>[2x]GPLGSKNHTLYDGQSNGEAKVKKIEFSEFTVKIKNKNNSNNWADLGDLVVRKEEDGIETGLNVGKGDSDTFAGYTATFFSLEESEVNNFIKAMTEGGSFKTSLYYGYKDEQSNANGIQNKEIITKIEKIDDFEYITFLGDKIKDSGDKVVEYAILLEDLKKNLK

The bacterium utilizes a set of proteins, termed complement regulator-acquiring surface proteins (CRASPs), to aid evasion of the human complement system by recruiting and presenting complement regulator factor H on its surface in a manner that mimics host cells. Another member of the CRASP family, ErpC (also referred to as BbCRASP-4), is an 18 kDa protein that belongs to the OspE/F-related (Erp) paralogous family of proteins and has also been demonstrated to bind factor H. Moreover, ErpC has been implicated in the scavenging of complement factor H-related proteins CFHR-1, CFHR-2 and CFHR-5, although the functional implications of this ability to bind multiple complement proteins has yet to be fully understood. ErpC is a member of the CRASP family of proteins which aid in complement evasion by B. burgdorferi by binding and presenting complement factor H on the bacterial cell surface under distinct circumstances.

The atomic resolution structure of ErpC has been solved, showing the formation of a β-­barrel, an architecture which is completely different to the pre­dominantly α-helical CspA, which is the only other member of the CRASP family for which the structure has been elucidated. Several of the loops between β-strands could not be built in one or both copies of ErpC in the unit cell owing to a lack of electron density, suggesting that these regions are conformationally labile. However, ErpC lacks the additional structural elements that are involved in these assemblies, suggesting that it does not multimerize in a similar manner, and analysis of the interfaces between the ErpC molecules in the crystal using PISA suggested that there were no biologically relevant assemblies. The observed molecular mass of 17 000 Da correlated with the expected molecular mass of ErpC (18 316 Da), confirming that the protein is monomeric under these conditions and, in conjunction with the PISA analysis, that it is likely to be monomeric on the spirochete surface. The solvent-accessible surface of ErpC exhibits large regions of negative charge, which suggests that ErpC may be acting in a similar capacity by binding factor H via interaction interfaces reserved for host-cell localization. The binding site of complement regulators on ErpC is likely to involve residues within the loops between the β-strands in a similar manner to other bacterial factor H-binding proteins. Mapping the sequence conservation between ErpC, its paralogue OspE and members of the OspE/F-related protein family, including ErpP and ErpA, across different B. burgdorferi strains reveals that variation occurs mainly within these loops. These findings suggest that ErpC, ErpP, ErpA and OspE share a common architecture and are individually tailored to binding specific complement proteins with different affinities.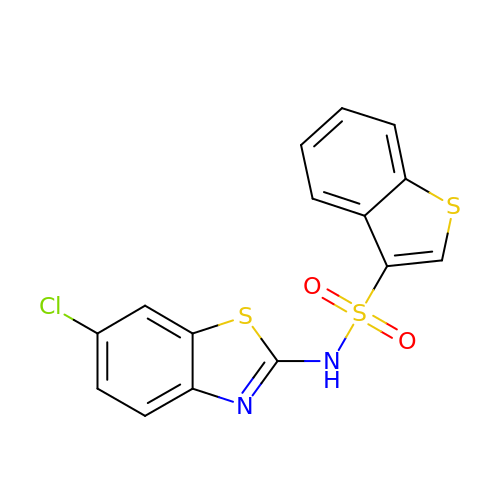N-(6-chloro-1,3-benzothiazol-2-yl)-1-benzothiophene-3-sulfonamide | C15 H9 Cl N2 O2 S3 | VLGMTYRMKMVUHJ-UHFFFAOYSA-N>VEGRFQLVAPYEPQGDQPQAIAKLVDGLRRGVKHQTLLGATGTGKTFTISNVIAQVNKPTLVIAHNKTLAGQLYSELKEFFPHNAVEYFVCYYDYYQPEAYVPQTDTYIEKDAKINDEIDKLRHSATSALFERRDVIIVASVSSIYGLGSPEEYRELVVSLRVGMEIERNALLRRLVDIQYDRNDIDFRRGTFRVRGDVVEIFPASRDEHSIRVEFFGDEIERIREVDALTGEVLGEREHVAIFPASHFVTREEKMRLAIQNIEQELEERLAELRAQGKLLEAQRLEQRTRYDLEMMREMGFSSGIENYSRHLALRPPGSTPYTLLDYFPDDFLIIVDESHVTLPQLRGMYNGDRARKQVLVDHGFRLPSALDNRPL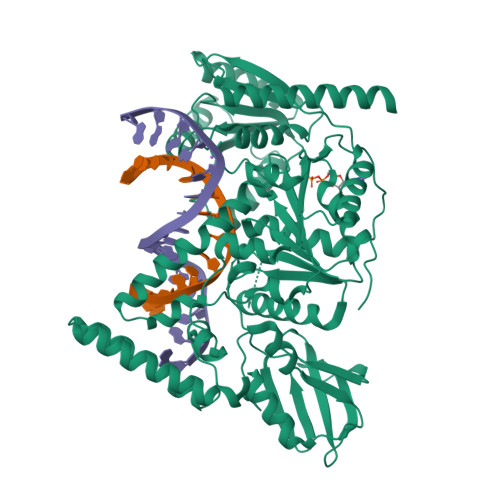TFEEFEQKINQIIYVSATPGPYELEHSPGVVEQIIRPTGLLDPTIDVRPTKGQIDDLIGEIRERVERNERTLVTTLTKKMAEDLTDYLKEAGIKVAYLHSEIKTLERIEIIRDLRLGKYDVLVGINLLREGLDIPEVSLVAILDADKEGFLRSERSLIQTIGRAARNANGHVIMYADTITKSMEIAIQETKRRRAIQEEYNRKHGIVPRTVKKEIR[3x]> MSCVYAFGSNGQR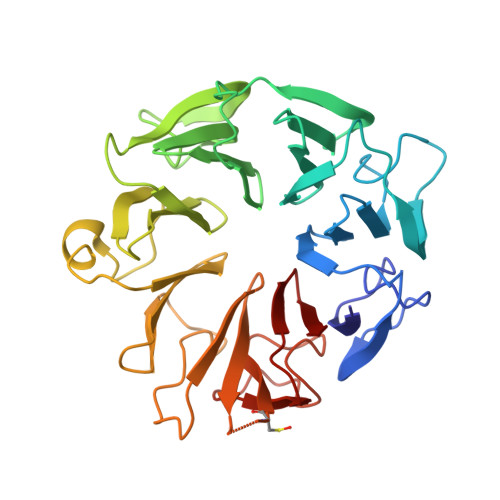QLGLGHDEDMDTPQRSVPGDDGAIVRKIACGGNHSVMLTNDGNLVGCGDNRRGELDSAQALRQVHDWRPVEVPAPVVDVACGWDTTVIVDADGRVWQRGGGCYEFTQQHVPLNSNDERIAVYGCFQNFVVVQGTRVYGWGSNTKCQLQEPKSRSLKEPVLVYDTGSVAVDYVAMGKDFMVIVDEGGRIVHASGRLPTGFELKQQQKRHNLVVLCMWTSIHLWNARLNTVESFGRGTHSQLFPQERLDFPIVGVATGSEHGILTTANQEGKSHCYNVYCWGWGEHGNCGPQKGSQPGLQLVGQYSGKPRVFGGCATTWIVL(3R,4E)-4-[({3-hydroxy-2-methyl-5-[(phosphonooxy)methyl]pyridin-4-yl}methyl)imino]cyclopent-1-ene-1,3-dicarboxylic 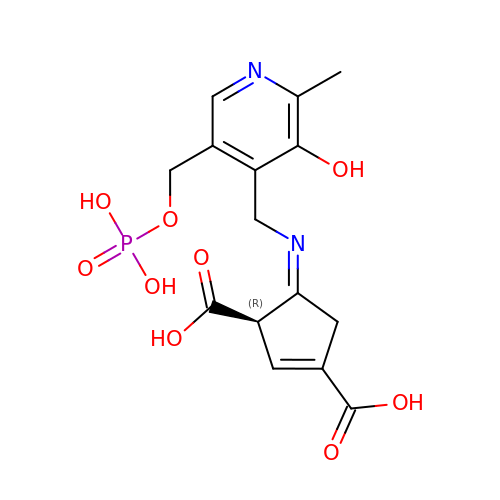acid | C15 H17 N2 O9 P | ZCYQKEUHCZMBPP-IDWSFWJTSA-N> MLRINGTFLYDRRWADEEKIMETKSLSESTICCFGDSTTWGDNGCGGGGNDISWTSHLGALLGGAVVENFGIKGSRIAIKADRTDSFVERLDGIDDAADVYVVFGGVNDFSRNVPLGELGSTDAHEFYGAVDYLIRTITARSPQAKLVFMTPCKTSGKHEKDIPASDELNHLGLTQAAYVRAMLEVCDRYSVPVIDLYAQSGISPFLPEHRELYMP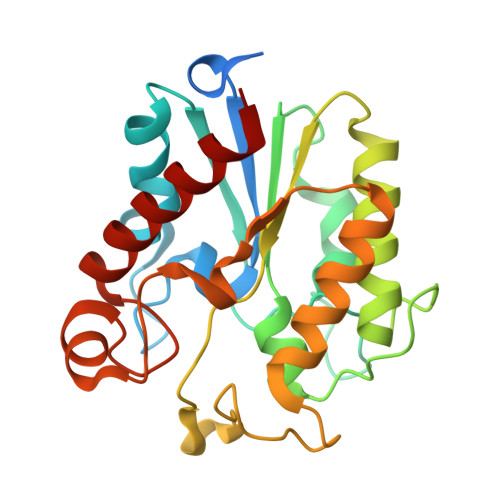DGLHYSPAGYERLAHRIAAGLTAVCR>GHMPKVIDKATPYADLLVPKLAMSVKDGAVGVAVDAPVTVTAGEGVLGSVTMVNSDGKEIAGEIGPDGVTWTTTEPLGYDKQYTINADARGLGGVARANATFRTQSPDNMTMPYVMPGDGEVVGVGQTVAIRFDENIPNRAAAEKAIKITTNPPVEGAFYWLNNREVRWRPESFWDSGTSVDVKVNTYGVNLGDGVFGQDNVASHFTIGDAVISRVDDTNKILNIERNGEIIKTMPTSMGKDKAPTNNGTYIIGERFKDLIMDSST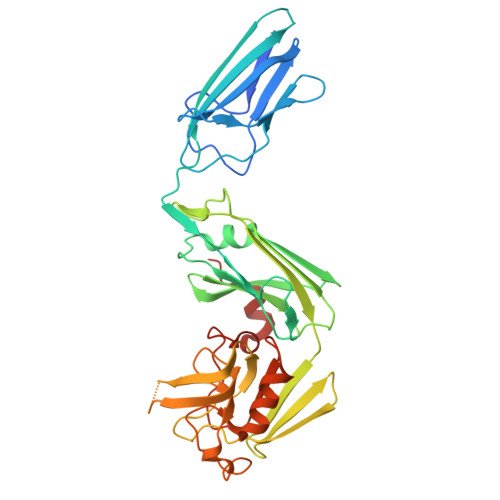YGVAVNSPDGYRTKVQYATQMSYSGIYVHAAPWSVGAQGRTNTSHGCLNVSTANAKWFYENTKRGDVVIVSNTVGPVLPGTEGLGDWNIPWAQWKAGNARQQ[6x]>APLAPASYHPKPWLGAQPATVVTPGVNVTLRCRAPQPAWRFGLFKPGEIAPLLFRDVSSELAEFFLEEVTPAQGGSYRCCYRRPDWGPGVWSQPSDVLELLVTEELPRPSLVALPGPVVGPGANVSLRCAGRLRNMSFVLYREGVAAPLQYRHSAQPWADFTLLGARAPGTYSCYYHTPSAPYVLSQRSEVLVIAAA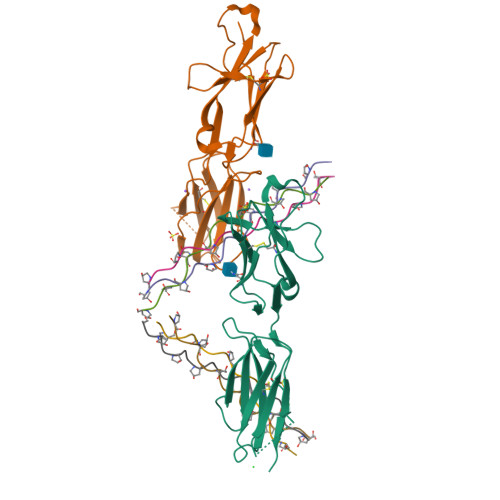HHHHHH[2x];>GPPGPPGPPGPAGFPGPPGPP[6x];>PGPPGPP[3x]>RDPDLEIRAAFLEKENTALRTEVAELRKEVGRCKNIVSK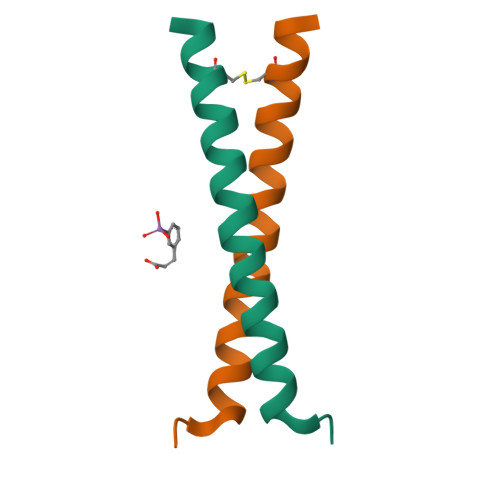[2x]>[2x]EEAKLTAHYSFDNNDLSDSTGNFGPGTITGNRIDNEGGTIAYADGKIGKAAVLNGQSGIRLPDG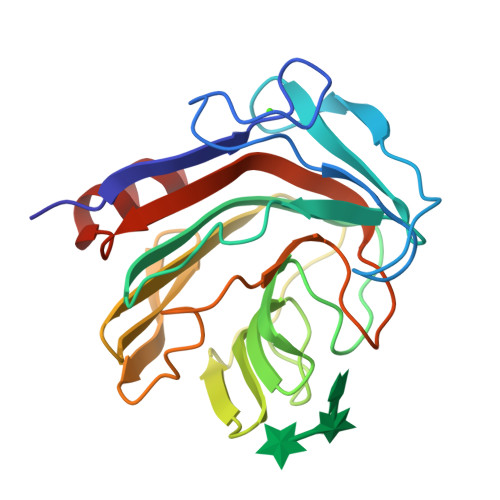LVSSNQYSVSLWVKPEQLTTHTTTFFGAKDPNHWISLVPQGWDGNTMLWSGSSPWYDGRTFWKIPTGQWTHLAFSVDNGAVKVYINGVEKFSGTNFPDVFTGANASFALGVNWWDPPFKGLIDELRIYEGALTPSQVTDLAQTSE>[12x]MAEQTEQTTTPFVLPGLNYVHSGFPAPGLRQINRHITGHDD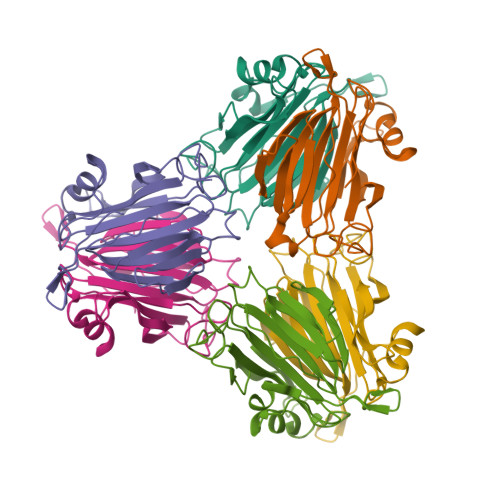NGKSVFLSTDHGDHHRIMGEKQAVANILYSTQETPVQLNGNVDIDKAAKEEPPLHYHNGSIVRMIDFAPAVESPLHRAVSIDYGIVVEGVFKLVLDSGEERIMRQGDVSVQRATAHKWINITDNGTAPGRMMWILLDCHDVVVNGQVMEGYLGDLEKEYVGRGASK>[2x]NTTIESIGNNNQQWPIPLTGVPVGDFYVYGRMTTLHMGGQSGIQATTLVNGMIYRTDHPEPSTSPVSNWEFTVLENNTIVGAGMGCVWFQKSEVLVWTLDGQKLSGWNTL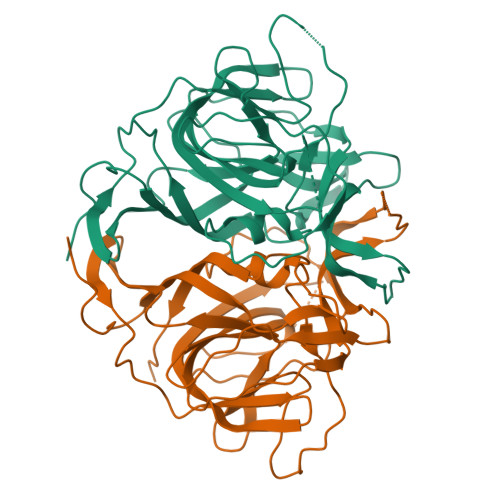DGVGTTQLTVAWRQHNRTIYGWANVVAWNSEEWHTNAERLHQPTLRLTYWLVKINVSSEPEDFDVVQKFPLAYLEDYTTAQSKSAIQKLNFQTFQKPEGGGTLRAQYSTVPRQGDFAVIWQIGRHNFDMSTGKGTPVESLSDYVMPEQKDARIGMWYRALTSVGPRSDMLTLHFHFPTVEKDLVEQIIDQIQHR4-amino-2-[(1,3-dimethyl-1H-pyrazol-4-yl)amino]-7-methyl-6-[(2R)-2-methylpyrrolidin-1-yl]-7H-pyrrolo[2,3-d]pyrimidine-5-carbonitrile 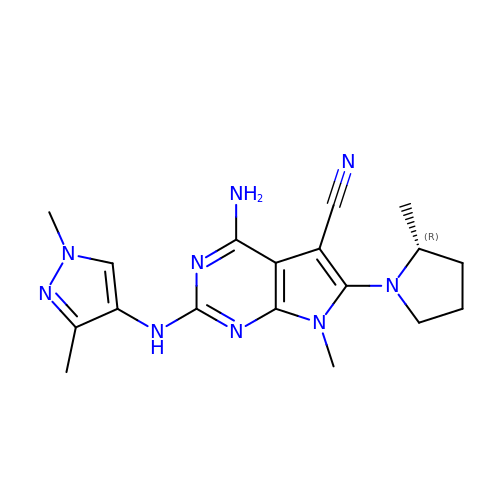| C18 H23 N9 | HZCHVYOFMPDLIU-SNVBAGLBSA-N> KPAFSKDDILPMDLGTFYREFQNPPQLSSLSIDIGAQSMAEDLDS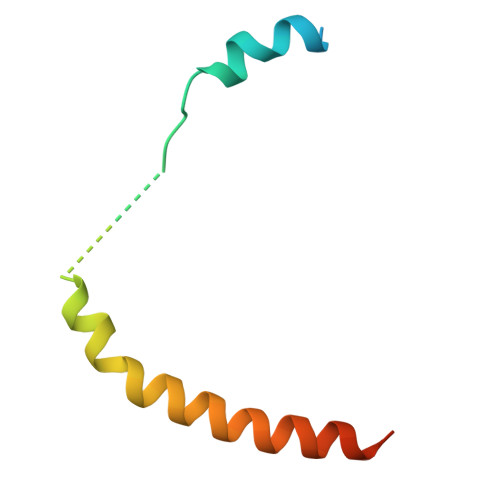LPEKLAVHEKNVREFDAFVETLQGSDEA>SMSEATPCIKAISPSEGWTTGGATVIIIGDNFFDGLQVVFGTMLVWSELITPHAIRVQTPPRHIPGVVE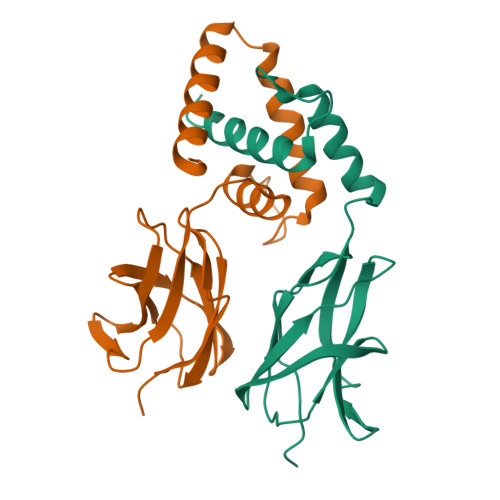VTLSYKSKQFCKGAPGRFVYTALNEPTIDYGFQRLQKVIPRHPGDPERLPKEVLLKRAADLVEALYGMPHNNQEIILKRAADIAEALYSV[6x]>MTSPSHASDRGGGDGDSVENQSPELRKDPVTNRWVIFSPARAKRPTDFKSKSPQNPNPKPSSCPFCIGREQECAPELFRVPDHDPNWKLRVIENLYPALSRNLETQSTQPETGTSRTIVGFGFHDVVIESPVHSIQLSDIDPVGIGDILIAYKKRINQIAQHDSINYIQVFKNQGASAGASMSHSHSQMMALPVVPPTVSSRLDGTKDYFEETGKCCLCEAKSKHFVIDESSHFVSVAPFAATYPFEIWIIPKDHSSHFHHLDDVKAVDLGGLLKLMLQKIAKQLNDPPYNYMIHTSPLKVTESQLPYTHWFLQIVPQLSGVGGFEIGTGCYINP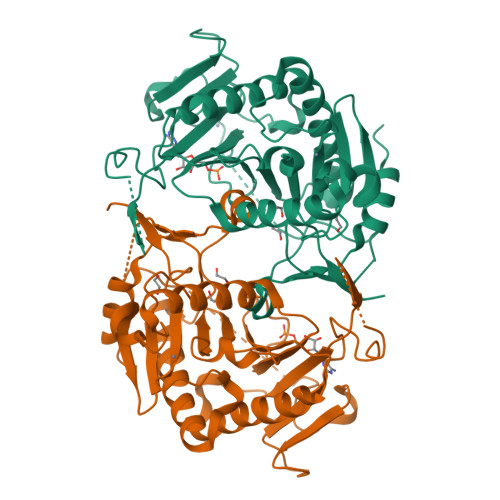VFPEDVAKVMREVSLT[2x]>[3x]GHMKDLKGTKTAENLKQGFIGESMANRRYLYFAK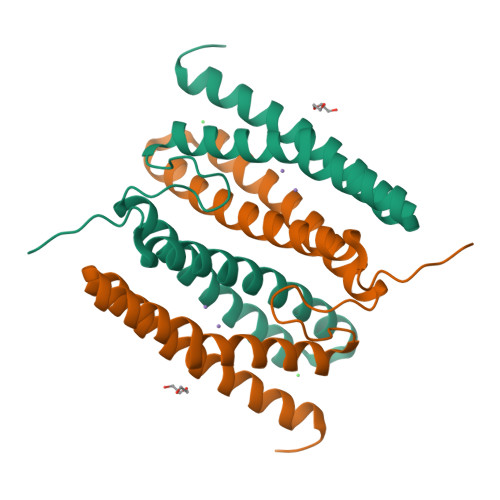RADEEGYPEIAGLLRSIAEGETAHAFGHLDFIRQGGLTDPATDKPIGTLEQMIESAIAGETYEWTQMYPGFAKVAREEGFPEVAEWFETLARAEKSHAEKFQNVLKQLKGGT> KYKLVFLGEQAVGKTSIITRFMYDTFDNNYQSTIGIDFLSKTLYLDEGPVRLQLWDTAGQ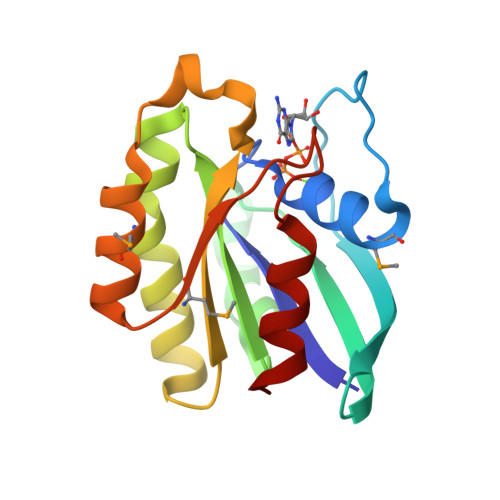ERFRSLIPSYIRDSAAAIVVYDITNRQSFENTTKWIQDILNERGKDVIIALVGNKTDLGDLRKVTYEEGMQKAQEYNTMFHETSAKAGHNIKVLFKKTASKL> SMPSQQRVKRWGFSFDEILKDQVGRDQFLRFLESEFSSENLRFWLAVQDLKKQPLQDVAKRVEEIWQEFLAPGAPSAINLDSHSYEITSQNVKDGGRYTFEDAQEHIYKLMKSDSYARFLRSNAY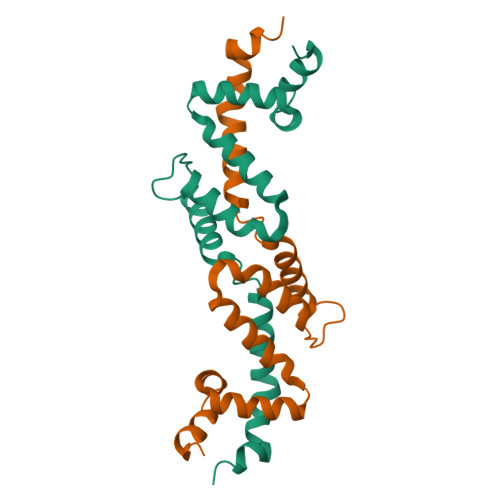QDLLLAKKKGKSLAGKRLTGLMQ> EFGTLVHDEQFIPDHILRVSVAQVPSACENREDVVVNGTSPGPAIHLLPGARTWIRVYNDMNDRNLSMHWHGLSQRFAPFSDGTPSATQWPIPPGHFFDYEILTEPEDAGTYFYHSHVGMQALSCTGPLIVEDCGSSPYHYDDERILLFQDHFQKSDLEMIQGLTSTQFTWTGETRGILLNGRGVSPNQAAVQGRPGEASGFFGSHRFSNFRAGDGTSNSWDGIRGDDQIEPPTDCTLPVIDVEPGKTYRLRFIGATGLSLLTMGFEDHNDLTIVQVDGSEYNAPVTVDHIQLGGGQRFDVLLRTKTAEELRCNGDKTTYFLQFETRDRPDPYRGYGVLRYNLGTPVPAAPTTPALTLPAEVNNWLEYTFQPLHPSSSLSPTAEEVTRRVILEAEQKIDPATGRLVWKLAHMTWTDMSRDKPVLVDIYERGEAAMPDYAAALTNYGWDPATKLFPAKKDEVLEIVIQNTGSHYSGASGIVETHPFHAHGQHFYDVGSGPGKYDPEANNAKLASLGYRPIKRDTTMVYRYGEGKVAPGEPAGWRAWRMKMNNPGVWMVHCHILAHMIMGMETIWVVGDAEDIVTIPLSVSQNYFTYGGSVYGNDTHAPEVYHYFDDTNKCCAAGAGDSEDSGHLEQKLISEEDLNSAVDHHHHHH

Multicopper oxidases are promiscuous biocatalysts with great potential for the production of industrial compounds. This study is focused on the elucidation of the structure–function determinants of a novel laccase-like multicopper oxidase from the thermophilic fungus Thermothelomyces thermophila (TtLMCO1), which is capable of oxidizing both ascorbic acid and phenolic compounds and thus is functionally categorized between the ascorbate oxidases and fungal ascomycete laccases (asco-laccases). Like common laccases, LMCOs perform a four-electron oxidation of a wide variety of phenolic compounds with the concomitant reduction of a dioxygen molecule to two molecules of water. Two catalytic copper sites are identified: a type 1 (T1) copper site close to the region where substrate oxidation occurs, and a trinuclear cluster (TNC) formed by a single type 2 (T2) copper ion and a pair of type 3 (T3a and T3b) copper ions. An electron extracted from the oxidized molecule in the T1 site is shuttled through a sequence of three highly conserved amino acids (the HCH bridge) to the TNC, where reduction of a dioxygen molecule to water occurs.

The crystal structure of TtLMCO1, determined using an AlphaFold2 model due to a lack of experimentally determined structures of close homologues, revealed a three-domain laccase with two copper sites, lacking the C-terminal plug observed in other asco-laccases. A disulfide bond is formed between Cys28 and Cys236, stabilizing the relative orientation of domains A and B. In accordance with the bioinformatic analysis, the crystal structure revealed two N-glycosylation sites, including Asn37 [one N-acetylglucosamine (NAG) molecule] and Asn65 (two NAG molecules). In the T1 site, the copper ion is coordinated by the ND1 atoms of His564 (2.1 Å distance) and His483 (2.0 Å distance) and by the thiolate group of Cys559 (2.2 Å distance), forming a trigonal plane. Also, a methionine residue (Met569) is positioned axially to the T1 copper at a distance of 3.15 Å. A dioxygen molecule is modelled between the T3a and T3b coppers rather than a water molecule or a hydroxyl anion, since it fits more accurately into the ellipsoid shape of the electron density, while the peaks in the difference electron-density map disappear. The presence of a dioxygen molecule between the T3 coppers corresponds to the fully reduced state of the enzyme according to Polyakov et al.. The linear coordination of the T2 copper by the N atoms of His69 and His486 is a strong indication that the T2 copper is present in the reduced state. Furthermore, since the last 20 amino acids of TtLMCO1 were not included in the final structure due to a lack of electron density, there is no indication that the C-terminus of TtLMCO1 penetrates the T3 tunnel.> MNHKVHM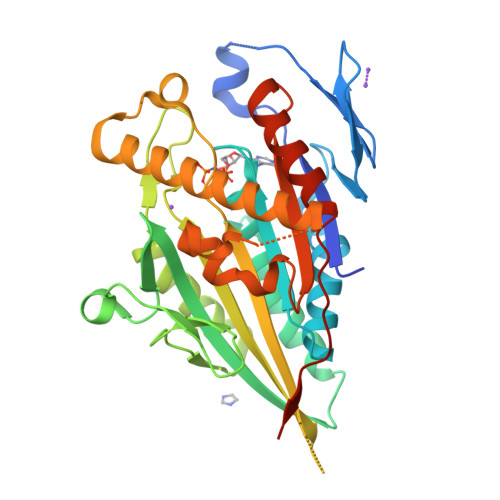AEEGAVAVCVRVRPLNSREESLGETAQVYWKTDNNVIYQVDGSKSFNFDRVFHGNETTKNVYEEIAAPIIDSAIQGYNGTIFAYGQTASGKTYTMMGSEDHLGVIPRAIHDIFQKIKKFPDREFLLRVSYMEIYNETITDLLCGTQKMKPLIIREDVNRNVYVADLTEEVVYTSEMALKWITKGEKSRHYGETKMNQRSSRSHTIFRMILESREKGEPSNCEGSVKVSHLNLVDLAGSERAAQTGAAGVRLKEGCNINRSLFILGQVIKKLSDGQVGGFINYRDSKLTRILQNSLGGNPKTRIICTITPVSFDETLTALQFASTAKYMKNTPYVNEVSGSHHHHHH2-(2-azanylethylamino)-5-nitro-benzoic 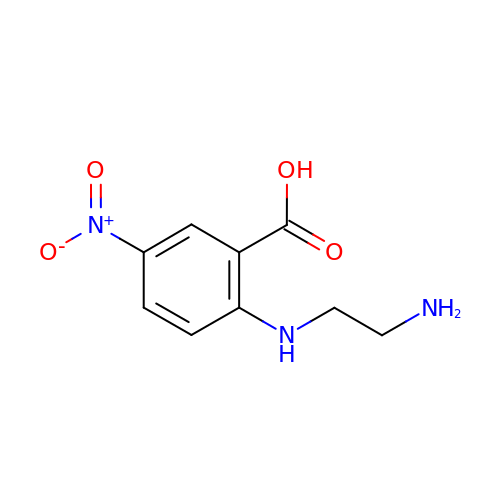acid | C9 H11 N3 O4 | PGIQBPZLZVDGHP-UHFFFAOYSA-N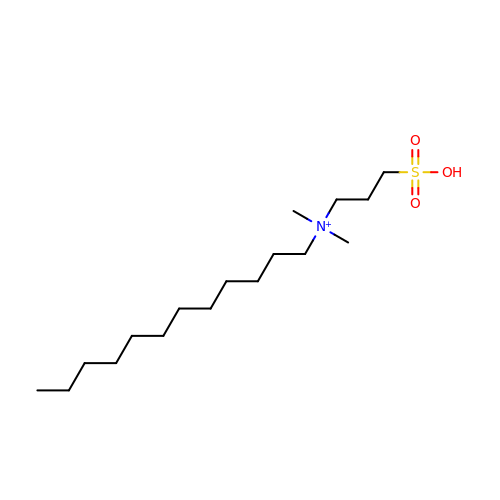N-DODECYL-N,N-DIMETHYL-3-AMMONIO-1-PROPANESULFONATE | C17 H38 N O3 S | IZWSFJTYBVKZNK-UHFFFAOYSA-O> MDPDQYSIEADKKFKYSLKLSDYPTLQDAASAAVDGLLIDRDYNFYGGETVDFGGKVLTIECKAKFIGDGNLIFTKLGKGSRIAGVFMESTTTPWVIKPWTDDNQWLTDAAAVVATLKQSKTDGYQPTVSDYVKFPGIETLLPPNAKGQNITSTLEIRECIGVEVHRASGLMAGFLFRGCHFCKMVDANNPSGGKDGIITFENLSGDWGKGNYVIGGRTSYGSVSSAQFLRNNGGFERDGGVIGFTSYRAGESGVKTWQGTVGSTTSRNYNLQFRDSVVIYPVWDGFDLGADTDMNPELDRPGDYPITQYPLHQLPLNHLIDNL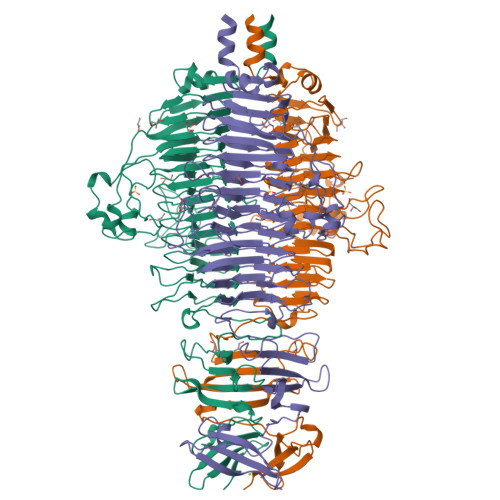LVRGALGVGFGMDGKGMYVSNITVEDCAGSGAYLLTHESVFTNIAIIDTNTKDFQANQIYISGACRVNGLRLIGIRSTDGQSLTIDAPNSTVSGITGMVDPSRINVANLAEEGLGNIRANSFGYDSAAIKLRIHKLSKTLDSGALYSHINGGAGSGSAYTQLTAISGSTPDAVSLKVNHKDCRGAEIPFVPDIASDDFIKDSSCFLPYWENNSTSLKALVKKPNGELVRLTLATL>[6x]MEIERINEHTVKFYMSYGDIEDRGFDREEIWYNRERSEELFWEVMDEVHEEEEFAVEGPLWIQVQALDKGLEIIVTKAQLSKDGQKLELPIPEDKKQEPASEDLDALLDDFQKEEQAVNQEEKEQKLQFVLRFGDFEDVISLSKLNVNGSKTTLYSFENRYYLYVDFCNMTDEEVENQLSILLEYATESSISIHRLEEYGKLIISEHALETIKKHFAS;>[6x]MMFGRFTERAQKVLALAQEEALRLGHNNIGTEHILLGLVREGEGIAAKALQALGLGSEKIQKEVESLIGRGQEMSQTIHYTPRAKKVIELSMDEARKLGHSYVGTEHILLGLIREGEGVAARVLNNLGVSLNKARQQVLQLLGSNETGSSAAGTNSNANTPTLDSLARDLTAIAKEDSLDPVIGRSKEIQRVIEVLSRRTKNNPVLIGEPGVGKTAIAEGLAQQIINNEVPEILRDKRVMTLDMGTVVAGTKYRGEFEDRLKKVMDEIRQAGNIILFIDELHTLIGAGGAEGAIDASNILKPSLARGELQCIGATTLDEYRKYIEKDAALERRFQPIQVDQPSVDESIQILQGLRDRYEAHHRVSITDDAIEAAVKLSDRYISDRFLPDKAIDLIDEAGSKVRLRSFTTPPNLKELEQKLDEVRKEKDAAVQSQEFEKAASLRDTEQRLREQVEDTKKSWKEKQGQENSEVTVDDIAMVVSSWTGVPVSKIAQTETDKLLNMENILHSRVIGQDEAVVAVAKAVRRARAGLKDPKRPIGSFIFLGPTGVGKTELARALAESIFGDEESMIRIDMSEYMEKHSTSRLVGSPPGYVGYDEGGQLTEKVRRKPYSVVLLDAIEKAHPDVFNILLQVLEDGRLTDSKGRTVDFRNTILIMTSNVGASELKRNKYVGFNVQDETQNHKDMKDKVMGELKRAFRPEFINRIDEIIVFHSLEKKHLTEIVSLMSDQLTKRLKEQDLSIELTDAAKAKVAEEGVDL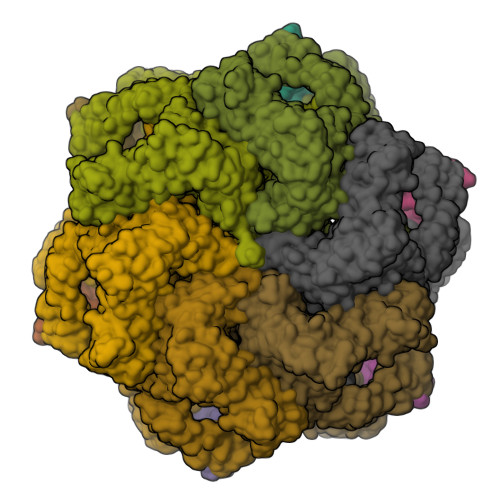EYGARPLRRAIQKHVEDRLSEELLRGNIHKGQHIVLDVEDGEFVVKTTAKTN Human dipeptidyl peptidase III (hDPP III), also known as enkephalinase B, is a member of the M49 family of zinc dependent metallopeptidases and cleaves dipeptides sequentially from the N-terminus of various bioactive peptide substrates. Crystal structures have so far been determined for DPP III from humans as well as from Saccharomyces cerevisiae. Despite the low sequence identity (36%) shared by the two proteins, both structures are very similar and consist of two lobes separated by a wide cleft. The “upper” lobe is mostly α-helical and contains the zinc binding site as well as the catalytically important residues. In both structures, two histidine residues (His-450 and His-455 in the human enzyme) and a glutamate (Glu-508) coordinate the zinc ion.

The octapeptide angiotensin-II (DRVYIHPF) is a potent vasoconstrictor and is involved in regulating mammalian blood pressure. Although angiotensin-II is not an opioid peptide, DPP III has been shown to cleave angiotensin-II in vitro. The dissociation constant (Kd) calculated from the ITC data was 1.64 μM. As in the previous examples, the N-terminus of the peptide forms extensive polar contacts with the conserved residues Asn-394, Glu-316 and Tyr-318 and is involved in β-type interactions with the core of the protein. The side chain of Asp-1 of the peptide forms a salt bridge with Arg-399 and is additionally hydrogen bonded to His-455 from the conserved HELLGH zinc-binding motif. His-568 interacts with the carbonyl of Arg-2 of angiotensin-II, again supporting the hypothesis of oxyanion stabilization during catalysis. The guanidinium group of Arg-572 forms hydrogen bonds with carbonyl groups of Tyr-4 and His-6 of angiotensin-II. In order to be accommodated in the binding cleft, angiotensin-II adopts a turn-like conformation with a cis-peptide formed between His-6 and Pro-7. Arg-669 forms a hydrogen bond with the carbonyl group of Ile-5, whereas Lys-670 forms a salt bridge with the C-terminal carboxylate of the ligand. It appears that the binding cleft is voluminous enough to accommodate a heptapeptide in a more or less extended conformation, whereas longer peptides have to bend as seen in the angiotensin-II complex.

> MADTQYILPNDIGVSSLDSREAFRLLSPTERLYAYHLSRAAWYGGLAVLLQTSPEAPYIYALLSRLFRAQDPDQLRQHALAEGLTEEEYQAFLVYAAGVYSNMGNYKSFGDTKFVPNLPKEKLERVILGSEAAQQHPEEVRGLWQTCGELMFSLEPRLRHLGLGKEGITTYFSGNCTMEDAKLAQDFLDSQNLSAYNTRLFKEVDGCGKPYYEVRLASVLGSEPSLDSEVTSKLKSYEFRGSPFQVTRGDYAPILQKVVEQLEKAKAYAANSHQGQMLAQYIESFTQGSIEAHKRGSRFWIQDKGPIVESYIGFIESYRDPFGSRGEFEGFVAVVNKAMSAKFERLVASAEQLLKELPWPPTFEKDKFLTPDFTSLDVLTFAGSGIPAGINIPNYDDLRQTEGFKNVSLGNVLAVAYATQREKLTFLEEDDKDLYILWKGPSFDVQVGLHALLGHGSGKLFVQDEKGAFNFDQETVINPETGEQIQSWYRCGETWDSKFSTIASSYEECRAESVGLYLSLHPQVLEIFGFEGADAEDVIYVNWLNMVRAGLLALEFYTPEAFNWRQAHMQARFVILRVLLEAGEGLVTITPTTGSDGRPDARVRLDRSKIRSVGKPALERFLRRLQVLKSTGDVAGGRALYEGYATVTDAPPESFLTLRDTVLLRKESRKLIVQPNTRLEGSDVQLLEYEASAAGLIRSFSERFPEDGPELEEILTQLATADARFW;> DRVYIHPF> MEKKKYTAPQLAKVGEFKEATG;> GPVSSKEQTVETTGAEFRLRPEISVAQTDYGMVLLDGRSGEYWQLNDTAALIVQRLLDGHSPADVAQF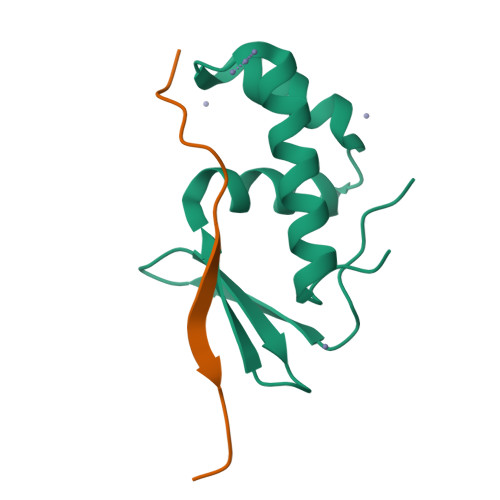LTSEYEVERTDAERDIAALVTSLKENGMALP> MGSDKIHHHHHHMGLSRVRAVFFDLDNTLIDT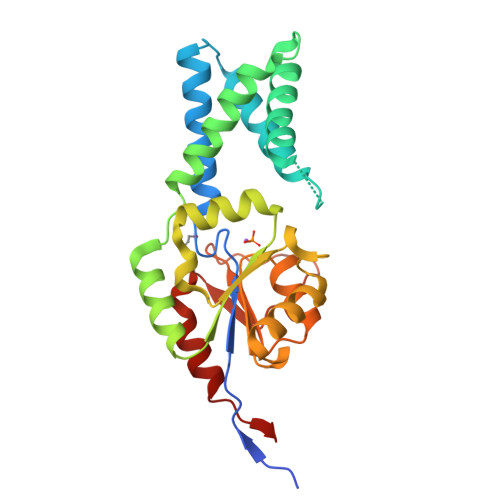AGASRRGMLEVIKLLQSKYHYKEEAEIICDKVQVKLSKECFHPYSTCITDVRTSHWEEAIQETKGGADNRKLAEECYFLWKSTRLQHMILADDVKAMLTELRKEVRLLLLTNGDRQTQREKIEACACQSYFDAIVIGGEQKEEKPAPSIFYHCCDLLGVQPGDCVMVGDTLETDIQGGLNAGLKATVWINKSGRVPLTSSPMPHYMVSSVLELPALLQSIDCKVSMSV> 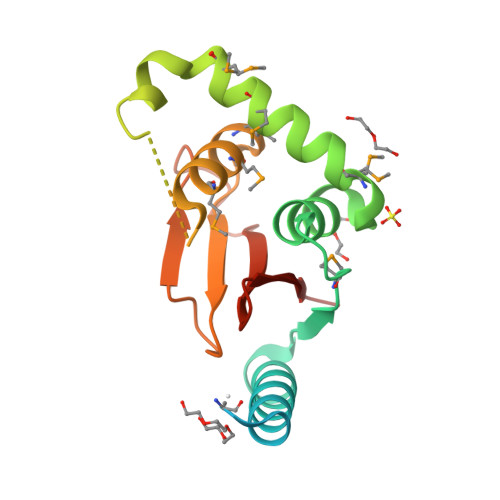MHHHHHHSSGRENLYFQGAGYNSEDEYEAAAARIEAMDPATVEQQEHWFEKALRDKKGFIIKQMKEDGACLFRAVADQVYGDQDMHEVVRKHCMDYLMKNADYFSNYVTEDFTTYINRKRKNNCHGNHIEMQAMAEMYNRPVEVYQYSTEPINTFHGIHQNEDEPIRVSYHRNIHYNSVVNPNKA> SMKRGRGGRVDPFEFVTYSGEEIKESSSEERVKEGANKSSPT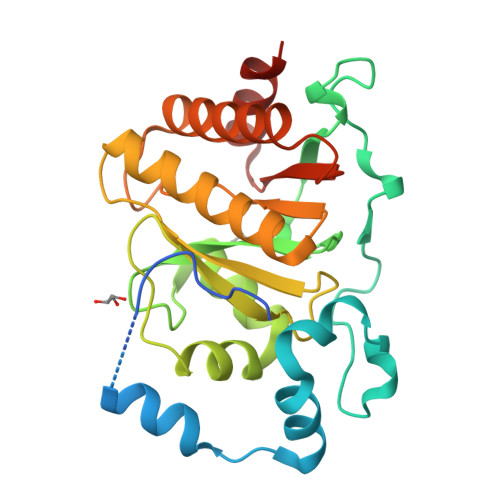RTRILSAALSPAERAIFDVPIEKWLSIDRSSLSGWKCAVPRPVTIEQLRPVDPSDAILRHIALYRGPVTDLQLDAIVNAANTRCLGGGGVDGAIHRVAGPLLLRECATFNGCQTGECRLTKGYQLPARYVLHTVGPVGERPDMLRKCYRSILSLALKNGLRSIGFCCVSTGVYGYPLLPATRIALGETRKFLEEHGGALDMCCFACFQEDEYKTYEKCVGKSSL>[2x]HHHHHHMSAKDERAREILRGFKLNWMNLRDAETGKILWQGTEDLSVPGVEHEAR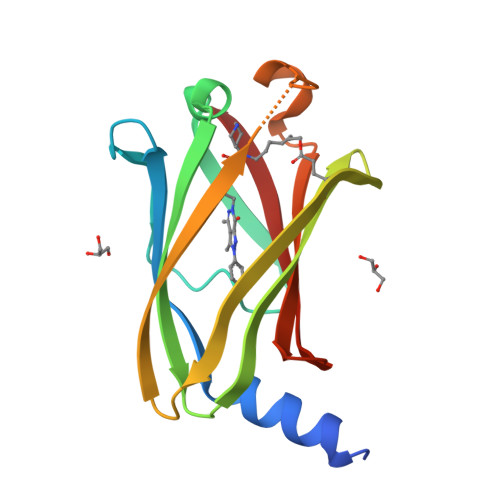VPKKILKCKAVSRELNFSSTEQMEKFRLEQKVYFKGQCLEEWFFEFGFVIPNSTNTWQSLIEAAPESQMMPASVLTGNVIIETKFFDDDLLVSTSRVRLFYV>MAPEAQVSVQPNFQQDKFLGRWFSAGLASNSSWLREKKAALSMCKSVVAPATDGGLNLTSTFLRKNQCETRTMLLQPAGSLGSYSYRSPHWGSTYSVSVVETDYDQYALLYSQGSKGPGEDFRMATLYSRTQTPRAELKEKFTAFCKAQGFTED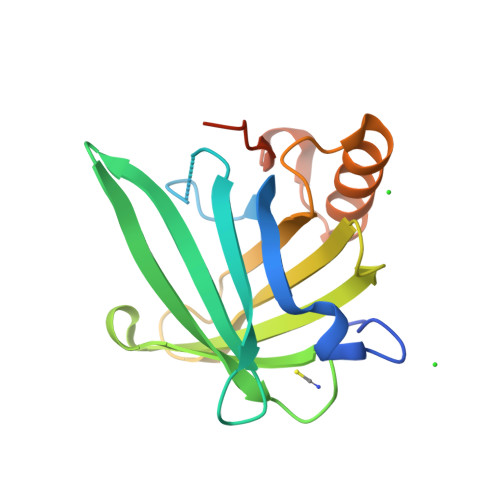TIVFLPQTDKCMTEQAHHHHHH[2x]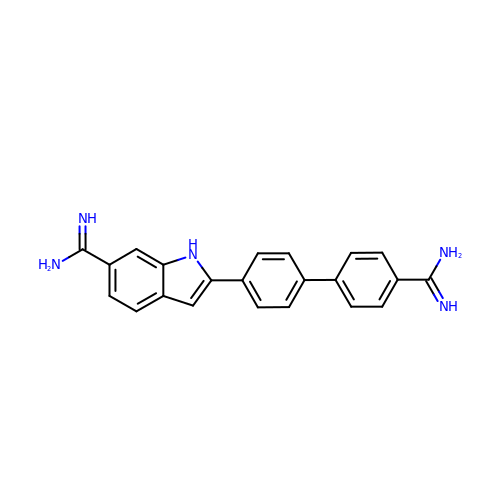2-(4'-carbamimidoylbiphenyl-4-yl)-1H-indole-6-carboximidamide | C22 H19 N5 | UCQUHTKKHKLNML-UHFFFAOYSA-N> MPSGTDDPLSDAEIQKYREEINRLDREILDAVKRRTKISQTIGKTRMSSG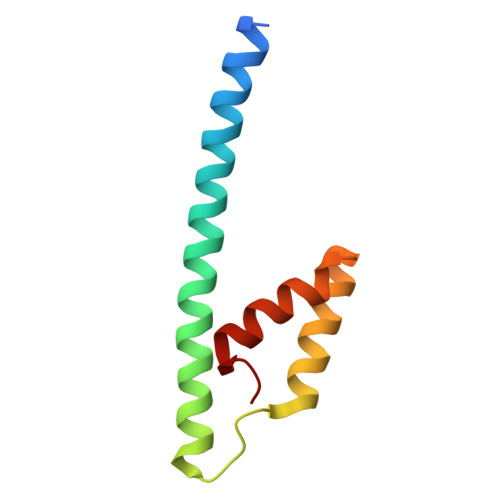GTRLVHTREVAIINQFREEIGEEGPALAGILLRMGRGKLG>[2x]MAHHHHHHVDDDDKMNS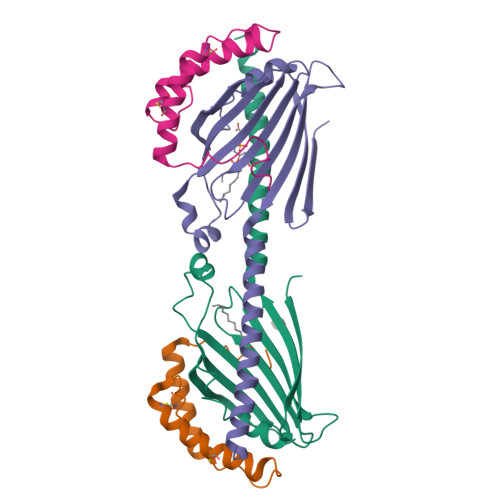VGEACTDMKREYDQCFNRWFAEKFLKGDSSGDPCTDLFKRYQQCVQKAIKEKEIPIEGLEFMGHGKEKPENSS;>GSSHHHHHHSDQMVKYFLGQSVLRSSWDQVFAAFWQRYPNPYSKHVLTEDIVHREVTPDQKLLSRRLLTVTNRMPRWAERLFPANVAHSVYVLEDSIVDPQNQTMTTFTWNINHARLMVVEERSVYSVNSDNSGWTEIRREAWVSSSLFGVSRAVQEFGLARFKSNVTKTMKGFEYILAKLQGEA[2x]>[6x]ADECPTDWKMFNGRCFLFNPLQLHWADAQESCMKE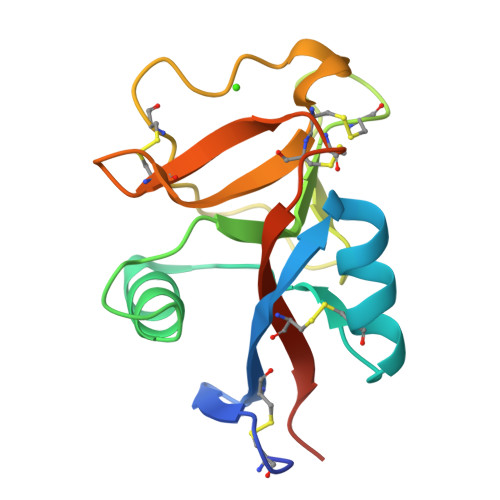GANLASIHSLEESTFVKELTSADLIPSWIGGTDCQVSTRWFWMDSTSMDYADWCAAQPDTTLTECCIQMNVGIGKCWNDTPCTHLHSSICAKPLKHHHHHH>MARCDVLVSADWAESNLHAPKVVFVEVDEDTSAYDRDHIAGAIKLDWRTDLQDPVKRDFVDAQQFSKLLSERGIANEDTVILYGGNNNWFAAYAYWYFKLYGHEKVKLLDGGRKKWELDGRPLSSDPVSRPVTSYTASPPDNTIRAF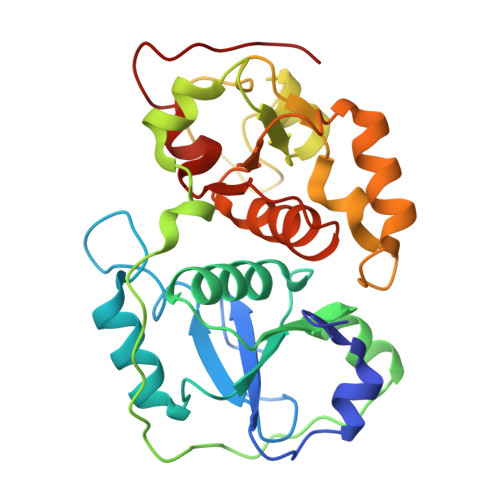RDEVLAAINVKNLIDVRSPDEFSGKILAPAHLPQEQSQRPGHIPGAINVPWSRAANEDGTFKSDEELAKLYADAGLDNSKETIAYCRIGERSSHTWFVLRELLGHQNVKNYDGSWTEYGSLVGAPIELGS[2x]Bacterial hybrid malic enzymes (MaeB grouping, multidomain) catalyse the transformation of malate to pyruvate, and are a major contributor to cellular reducing power and carbon flux. Distinct from other malic enzyme subtypes, the hybrid enzymes are regulated by acetyl-CoA, a molecular indicator of the metabolic state of the cell. The larger ME isoforms (hybrid enzymes) are predicted to be a fusion of two unrelated enzymes; a catalytic N-terminal ME subunit and a C-terminal phosphotransacetylase (PTA) domain. The PTA domain is homologous to PTA enzymes (that interconvert acetyl-CoA and phosphate to CoA and acetyl phosphate), yet they appear to lack critical catalytic residues and thus acts as a sensor instead.

As a control to mitigate any local/biased effects introduced by 3′ loop mutation, we designed a different unbound variant by mutation at the opposite end of the binding site—a N718D mutant repels ligand at the acetyl group. Supportively, N718D protein purifies without bound ligand and is also insensitive to inhibition. Interestingly, the N718D variant had increased activity compared to wt MaeB, indicative of release from inhibitor suppression. We were also able to generate structures for R535E, R535A and N718D PTA domain variants, which demonstrate the same features as the wt PTAapo structure.

>[12x]MGSSHHHHHHSSGLVPAGSHSKVFIRSAINRVHQNSAANGGELPRIVFPEGTSTKVLKALATLVEEKICQPILLGYPERVKEKIKALDIPLLNDVSIVHPSSHPKYFSFVEKLYSLRQRKGINLGEAERLMADPNYFAAMMVNQGEADGMVSGSSINYADAVRPILQTIGVYKEGIPAGLNFVLLEDKFLVLADTTVNLNPTAEQCAQIALQAAKIVEYFGIEPRVAMLSYSNFSGAEGTPRKMKKAAEIARSLRPDLMIEGDMQADTAVNPEIMERLFPFSGLKGGANVLVFPNLESSDIAYKLIQQIGKAEVIGPFLTGVRRSANVLQRTTTVDGIVNSVVFTALEAQYIKEVLKSRGKK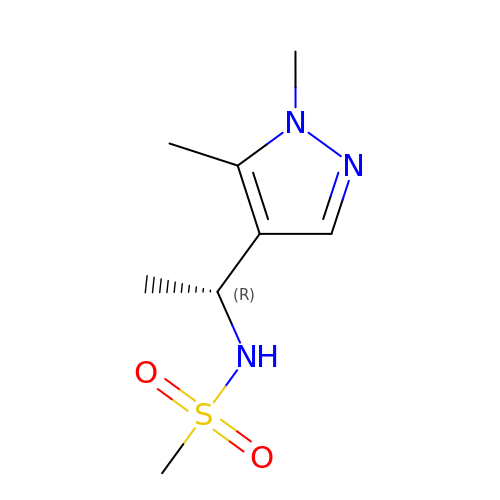N-[(1R)-1-(1,5-dimethyl-1H-pyrazol-4-yl)ethyl]methanesulfonamide | C8 H15 N3 O2 S | DPWJNSPPALAEBZ-UHFFFAOYSA-N6-(5,5,8,8-TETRAMETHYL-5,6,7,8-TETRAHYDRO-NAPHTALENE-2-CARBONYL)-NAPHTALENE-2-CARBOXYLIC ACID | C26 H26 O3 | 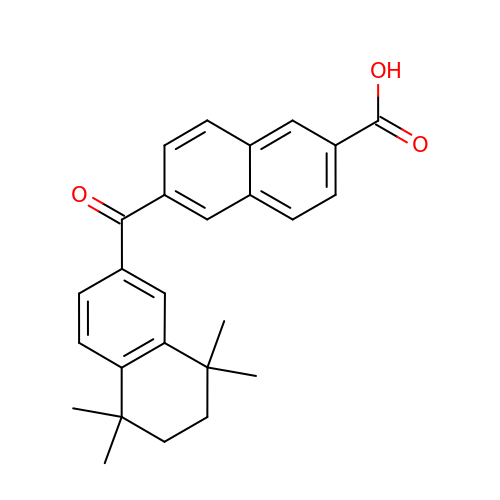RWYREGSYPCNZTL-UHFFFAOYSA-N[[1-[N-HYDROXY-ACETAMIDYL]-3-METHYL-BUTYL]-CARBONYL-LEUCINYL]-ALANINE 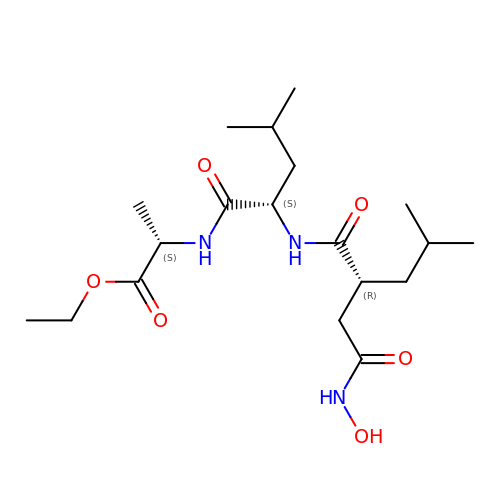ETHYL ESTER | C19 H35 N3 O6 | XKRONJXEXGFBRZ-ZNMIVQPWSA-N(2-{[(4-tert-butylphenyl)sulfonyl]carbamoyl}-5-methoxy-1H-indol-1-yl)acetic acid | C22 H24 N2 O6 S | 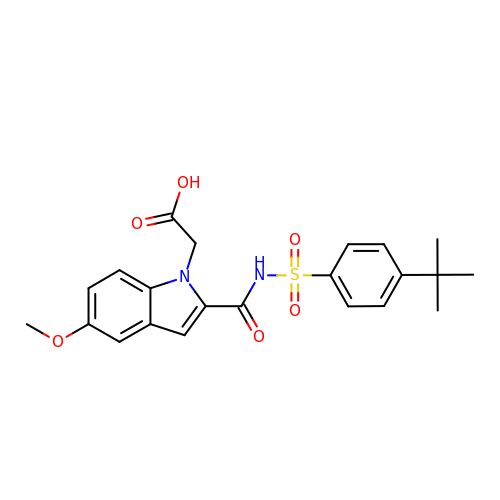MOBCJUUCVPLZOG-UHFFFAOYSA-N>QAQITGRPEWIWLALGTALMGLGTLYFLVKGMGVSDPDAKKFYAITTLVPPIAFTMYLSMLLGYGLTMVPFGGEQNPIYWARYADWLFTTPLLLLDLALLVDADQGTILALVGADGIMIGTGLVGALTKVYSYRFVWWAISTAAMLYILYVLFFGFTSKAESMRP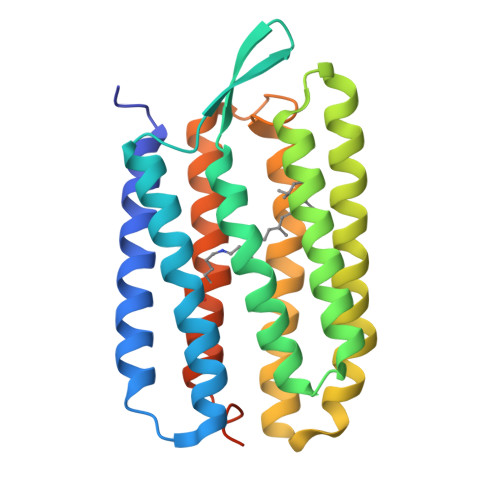EVASTFKVLRNVTVVLWSAYPVVWLIGSEGAGIVPLNIETLLFMVLDVSAKVGFGLILLRSRAIFGEAEAPEPSAGDGAAATSD[2x]>[2x]GSHMSQEEKLPKILIVEDDERLARLTQEYLIRNGLEVGV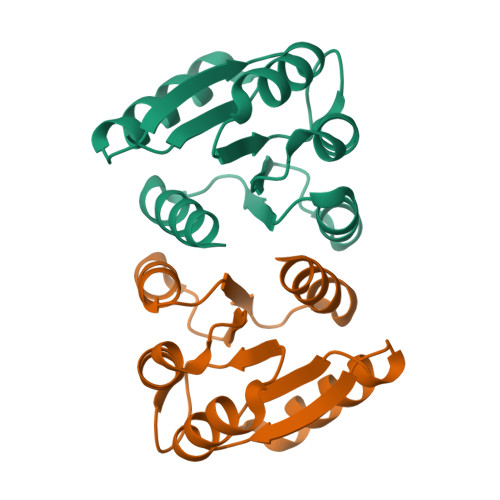ETDGNRAIRRIISEQPDLVVLDVMLPGADGLTVCREVRPHYHQPILMLTARTEDMDQVLGLEMGADDYVAKPVQPRVLLARIRALLRRTDKTVE> PELPEVETIRRTLLPLIVGKTIEDVRIFWPNIIRHPRDSEAFAARMIGQTVRGLERRGKFLKFLLDRDALISHLRMEGRYAVASALEPLEPHTHVVFCFTDGSELRYRDVRKFGTMH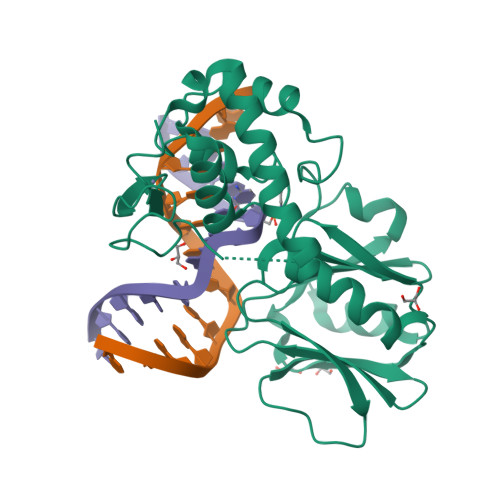VYAKEEADRRPPLAELGPEPLSPAFSPAVLAERAVKTKRSVKALLLDCTVVAGFGNIYVDESLFRAGILPGRPAASLSSKEIERLHEEMVATIGEAVMKGGSTVRTYVNTQGEAGTFQHHLYVYGRQGNPCKRCGTPIEKTVVAGRGTHYCPRCQR>MTAVRRIRAAALPDLPDASWSNALLVGEELVMSGMTAHPATRQAAERGAALDAHAQALVVLGKVKALLEAAGGHVGNLYKLNVYVTRIADKDAIGRARQEFFAGQGTFPASTLVEVSGLVFPELLVEIDAWA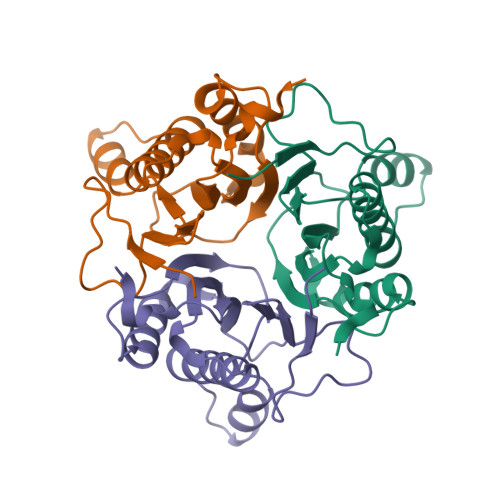RLDIDLANCDEA[3x]>MTGKT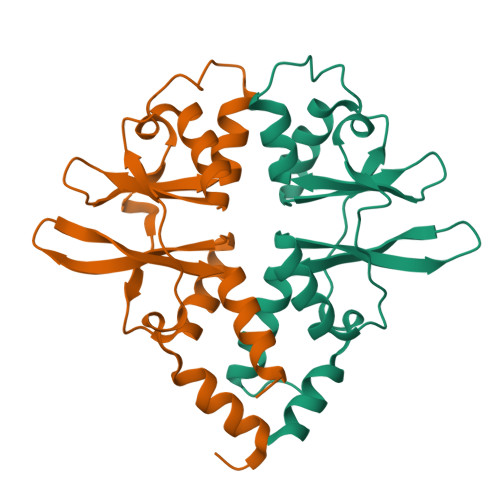GTQLLADKLKKLQVKDFQSIPVVIHENVSVYDAICTMFLEDVGTLFVVDRDAVLVGVLSRKDLLRASIGQQELTSVPVHIIMTRMPNITVCRREDYVMDIAKHLIEKQIDALPVIKDTDKGFEVIGRVTKTNMTKILVSLSENEILLQHHHHHH[2x]>MLDELVKKELSEEEITEIKLEEIIKYITLIKKSKTFVSSEIRKEELKFLSELAESLFELRLSKVLEGKVGKGFDEFIFDIFKILKQFYVDLLTGRYIIYNDKIYCIVQKPLIYNDHRVNEGDVLVLPMREALPLIIASYLTPYKIDIEEQL[2x];>MIEVKLRAIKRLSNVYTRRVMIIEDWNGSSITTGNIELVKGSENQLPQWLAIILEGKKVAKIEDKISIEDLGRILFQERQNMNTPASLVPLGKDFTSRVQLYLETLRKDNNVESLEKLRKSIGILNEIIKIRLRKLIQLAFLNIDDQNLINGMTEEELLIYKTIKQLIKELYGDIIGNS[2x]

Eukaryotes and archaea partly achieve this regulation by strictly controlling the activation of hexameric minichromosome maintenance (MCM) helicase rings that unwind DNA during its replication. In eukaryotes, MCM activation critically relies on the sequential recruitment of the essential factors Cdc45 and a tetrameric GINS complex at the onset of the S-phase to generate a larger CMG complex. Archaea also use a six-membered MCM ring to unwind DNA, and archaea possess GINS and Cdc45 homologs that stimulate the activities of MCM in biochemical DNA-unwinding assays. We present the crystal structure of the tetrameric GINS complex from the archaeal organism Saccharolobus solfataricus (Sso) to reveal a core structure that is highly similar to the previously determined GINS core structures of other eukaryotes and archaea.

The structure adopts a tetrameric architecture, with two copies of GINS51 and two copies of GINS23 in an approximately twofold-symmetric complex. Each subunit has two subdomains, with a larger α-helical subdomain (A) and a smaller subdomain that contains β-strands (B), consistent with the structures of other archaeal and eukaryotic GINS protein structures. The order of the A and B subdomains is reversed between the two subunits, with the A subdomain first in SsoGINS51 and the B subdomain first in SsoGINS23. In the archaeal structures, the core consists of both complete GINS23 subunits and the two GINS51A sub­domains. The underlying subdomain structure of GINS51B, Sld5B and Psf1B is conserved, but its placement relative to the GINS tetramer core varies among the structures. In the case of SsoGINS, the two GINS51B subdomains have a unique and sizable dimeric interaction surface. We therefore conclude that the dimeric interface of the SsoGINS51B subdomains of the crystal structure is not compatible with the simultaneous adoption of an interaction with polymerase as identified for TkGINS. Hence, the SsoGINS–RecJ interaction of the AlphaFold-Multimer model is consistent with the interactions observed in both archaea and eukaryotes and would not sterically clash with the conformation of the SsoGINS crystal structure. Although it is not known whether an SsoCMG structure would closely match eukaryotic CMG structures, this analysis shows that the 51B subdomain would need to move a large distance from its crystal structure position to accommodate a eukaryote-like CMG structure.3-CHLORO-N-((1R,2S) 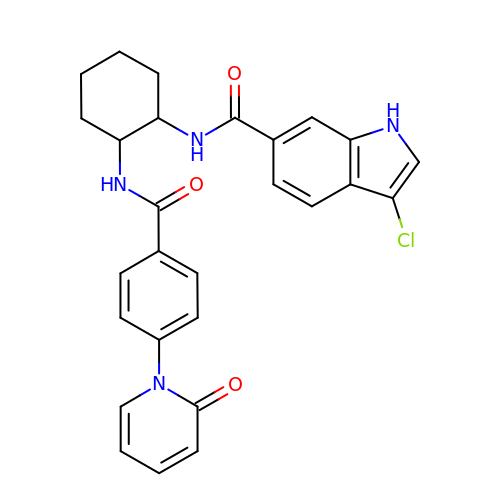-2-(4-(2-OXOPYRIDIN-1(2H)-YL)BENZAMIDO)CYCLOHEXYL)-1H-INDOLE-6-CARBOXAMIDE | C27 H25 Cl N4 O3 | PMRPPULYFDNTHJ-XZOQPEGZSA-N> KTEQPLSPYTAYDD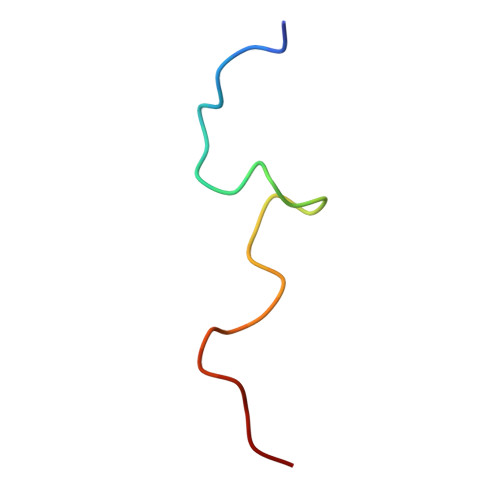LKPPSSPSPTKP> AASLAPGSSRVELFKRKNSTVPFEESNGTIRERVVHSFRIPTIVNVDGVMVAIADARYETSFDNSFIETAVKYSVDDGATWNTQIAIKNSRASSVSRVMDATVIVKGNKLYILVGSFNKTRNSWTQHRDGSDWEPLLVVGEVTKSAANGKTTATISWGKPVS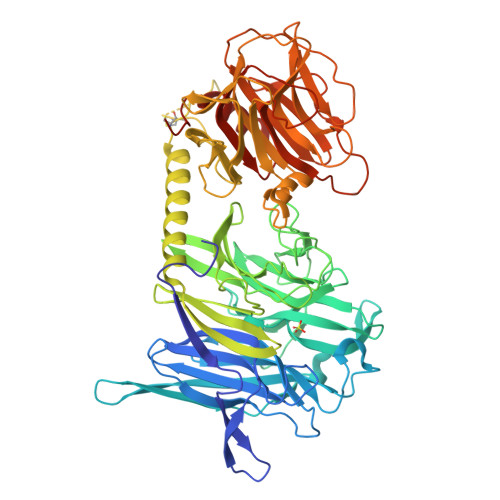LKPLFPAEFDGILTKEFVGGVGAAIVASNGNLVYPVQIADMGGRVFTKIMYSEDDGNTWKFAEGRSKFGCSEPAVLEWEGKLIINNRVDGNRRLVYESSDMGKTWVEALGTLSHVWTNSPTSNQQDCQSSFVAVTIEGKRVMLFTHPLNLKGRWMRDRLHLWMTDNQRIFDVGQISIGDENSGYSSVLYKDDKLYSLHEINTNDVYSLVFVRLIGELQLMKSVVRTWKEEDNHLASICTPVVPATPPSKGGCGAAVPTAGLVGFLSHSANGSVWEDVYRCVDANVANAERVPNGLKFNGVGGGAVWPVARQGQTRRYQFANYRFTLVATVTIDELPKGTSPLLGAGLEGPGDAKLLGLSYDKNRQWRPLYGAAPASPTGSWELHKKYHVVLTMADRQGSVYVDGQPLAGSGNTVVRGATLPDISHFYIGGPRSKGAPTDSRVTVTNVVLYNRRLNSSEIRTLFLSQDMIGTDGGAGTAA> GAGCAGCCTGTACGGACATCA;> CCGTACA;> GGCTGC;> CTTGATGT;> AGCCTACCTGCGTGGACAGAC;> CCACGCA;> G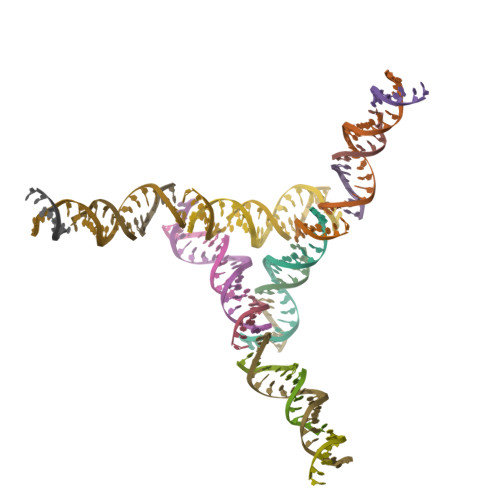GTAGG;> TCGTCTGT> MSEESQAFQRQLTALIGYDVTDVSNVHDDELEFTRRGLVTPRMAEVASRDPKLYAMHPWVTSKPLPEYLWKKIANNCIFIVIHRSTTSQTI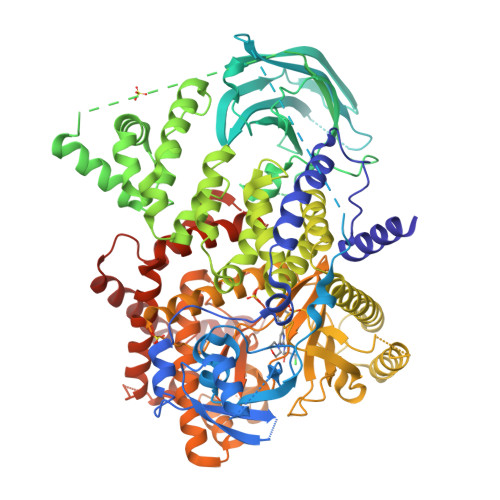KVSPDDTPGAILQSFFTKMAKKKSLMDIPESQSEQDFVLRVCGRDEYLVGETPIKNFQWVRHCLKNGEEIHVVLDTPPDPALDEVRKEEWPLVDDCTGVTGYHEQLTIHGKDHESVFTVSLWDCDRKFRVKIRGIDIPVLPRNTDLTVFVEANIQHGQQVLCQRRTSPKPFTEEVLWNVWLEFSIKIKDLPKGALLNLQIYCGKAPALSSKASAESPSSESKGKVQLLYYVNLLLIDHRFLLRRGEYVLHMWQISGKGEDQGSFNADKLTSATNPDKENSMSISILLDNYCHPIALPKHQPTPDPEGDRVRAEMPNQLRKQLEAIIATDPLNPLTAEDKELLWHFRYESLKHPKAYPKLFSSVKWGQQEIVAKTYQLLARREVWDQSALDVGLTMQLLDCNFSDENVRAIAVQKLESLEDDDVLHYLLQLVQAVKFEPYHDSALARFLLKRGLRNKRIGHFLFWFLRSEIAQSRHYQQRFAVILEAYLRGCGTAMLHDFTQQVQVIEMLQKVTLDIKSLSAEKYDVSSQVISQLKQKLENLQNSQLPESFRVPYDPGLKAGALAIEKCKVMASKKKPLWLEFKCADPTALSNETIGIIFKHGDDLRQDMLILQILRIMESIWETESLDLCLLPYGCISTGDKIGMIEIVKDATTIAKIQQSTVGNTGAFKDEVLNHWLKEKSPTEEKFQAAVERFVYSCAGYCVATFVLGIGDRHNDNIMITETGNLFHIDFGHILGNYKSFLGINKERVPFVLTPDFLFVMGTSGKKTSPHFQKFQDICVKAYLALRHHTNLLIILFSMMLMTGMPQLTSKEDIEYIRDALTVGKNEEDAKKYFLDQIEVCRDKGWTVQFNWFLHLVLGIKQGEKHSA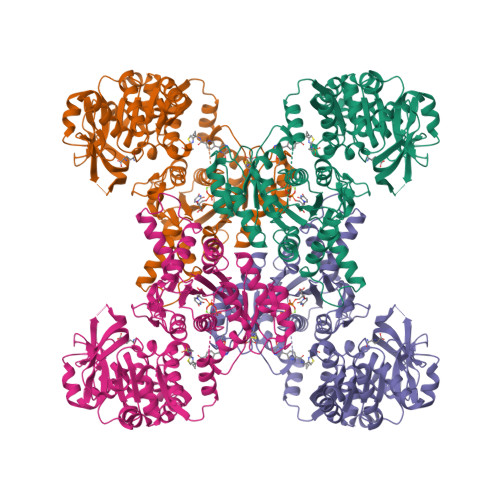>[4x]MKYILVTGGVISGIGKGVIASSVGTILKSCGLHVTSIKIDPYINIDAGTFSPYEHGEVFVLDDGGEVDLDLGNYERFLDIRLTKDNNLTTGKIYQYVINKERKGDYLGKTVQVVPHITDAIQEWVMRQALIPVDEDGLEPQVCVIELGGTVGDIESMPFIEAFRQFQFKVKRENFCNIHVSLVPQPSSTGEQKTKPTQNSVRELRGLGLSPDLVVCRCSNPLDTSVKEKISMFCHVEPEQVICVHDVSSIYRVPLLLEEQGVVDYFLRRLDLPIERQSRKMLMKWKEMADRYDRLLETCSIALVGKYTKFSDSYASVIKALEHSALAINHKLEIKYIDSTDLEPSTLQEEPVRYHEAWQKLCSAHGVLVPGGFGVRGTEGKIQAIAWARKQKKPFLGVCLGMQLAVVEFSRNVLGWQDANSTEFDPKTSHPVVIDMPEHNPGQMGGTMRLGKRRTLFQTKNSVMRKLYGDTDYLEERHRHRFEVNPVLKKCLEEQGLKFVGQDVEGERMEIVELEDHPFFVGVQYHPEFLSRPIKPSPPYFGLLLASVGRLPHYLQKGCRLSPRDTYSDRSGSSSPDSEITELKFPSISQD One specific mechanism used by nairoviruses is the production of a deubiquitinating enzyme, termed the vOTU, that disrupts the innate immune response. Interestingly, the nairoviral L segment also encodes a viral homologue of the ovarian tumor protease (OTU) at the N-terminus. Instead, the vOTU’s primary function appears to be the reversal of post-translational modifications by ubiquitin (Ub) and the Ub-like protein interferon stimulated gene product 15 (ISG15). Each vOTU possesses a seven-stranded beta sheet as the core feature, with five major alpha helices framing the rest of the structure.

The vOTUs from DGKV, QYBV, and TAGV readily crystallized and were solved to 1.62 Å, 1.65 Å, and 2.05 Å, respectively. These vOTUs represent diverse nairovirus species, and possess extensive variation in Ub activity with the DGKV, QYBV, and TAGV vOTUs possessing low, medium, and high activity towards Ub-AMC, respectively. In QYBV vOTU, Trp72 packs with Pro85. Additionally, it is in proximity to His79, suggesting potential stacking of the rings. In contrast, for QYBV vOTU there do not appear to be any direct interactions with the selectivity helix. Instead, Lys109 and Ser108 form electrostatic interactions with Asp15 and Asn16, respectively, suggesting a role in manipulating the positioning of the β1-β1a loop. Specifically, direct interactions, or the lack thereof, work in conjunction with the other interactions to complete the structural features. This is most notable in QYBV vOTU, in which Phe14 appears to pack with Pro76. In contrast, the DGKV and QYBV vOTUs possess more polar residues, including asparagine, glutamate, and threonine for DGKV and glutamine and lysine in QYBV. Despite being phylogenetically distant from CCHFV and the other robust vOTU DUBs, QYBV demonstrates substantial Ub activity and possesses Ile130 that could pack with Ub’s Leu8. Further, increasing the hydrophobicity of the pocket in QYBV vOTU was able to enhance Ub-AMC cleavage, boosting activity by 150% and 50% for the Q19V and Q128A mutants, respectively.

>[3x]MANLKENIVWEHVFDNCSQANVVFSYREFFNKELTLPDGNCFFRAVSTFLYDTQNGWIEVKNMCREFAETNWDELPGVHQYFQDPEHYARESKREGYWGGSVEAEILSKLLKLTVIFWKCEDDVWVTQGIRWGDGNYLTAINLLHIQFDHFDFLVPINVTQEPPKSGSHHHHHH> XTRT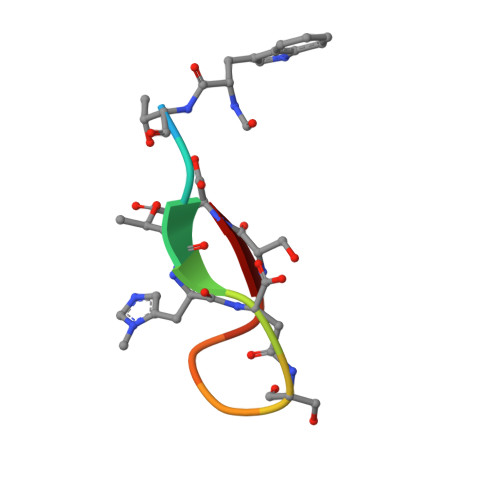XDSFGRSD>[2x]MATKTSIHPSVNELYQRLAEDQLSNCFDRFDPQEKIRCNYCELGVSCQL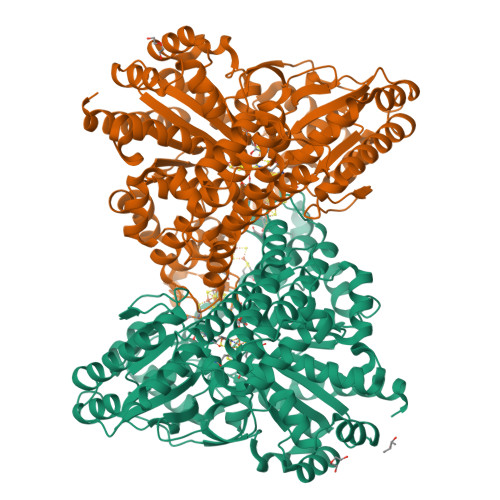CSNGPCRINEKVGATLGVCGINADGMAMRYMLLRNVMGTSTYTYHAYEAYKTLKMTALGNTPFTITDKDKLYQMAKDLELNTEGKPEDVAVRLSDFLIWELYRDYDEPGKMIEVYAPLKRKEVWRKLGIYPAGPLHELKDAAASCLTNVDGDYVSLATKGLRLGLSCIYGAQIGLELVQDILFGTGMPHEMDVDLGIFDADYINIVFNGHEPFVGVALILAAKEAVNQDKAKAAGAKSLRIYGSIESGQEVVQRFQKDEVFRGLTGNWLTIEPMLATGAVDVLAMDMNCSPPNLGPLAEKYGATLVSVSRLVRFPGIHHFLDYKPSEVREIAQKIIDIAVDSFKNKRHGKITPKIPANIQKAITGFTPEAILKALGGSINPLIEVIKAGKIKGAVGLINCTTLKNGPQDYVTVNLAKELIKRDILILSGGCGNHALEVAGLCNLDAINLAGPGLSEVCRNLNIPPVLSFGTCTDTGRISLVVTALANALNVDTADLPVAVTAPMYMEQKATIDALFALAYGLYTHVAPDPPVMGAPNLVKLLTRDLPSITGGRIAVGSDPVKVADDILAHINDRRAKLGI> NSPLHTVGFDARFPQQNQTKHCWQSYVDYHKCVNMKGEDFAPCKVFWKTYNALCPLDWIEKWDDQREKGIFAGDINS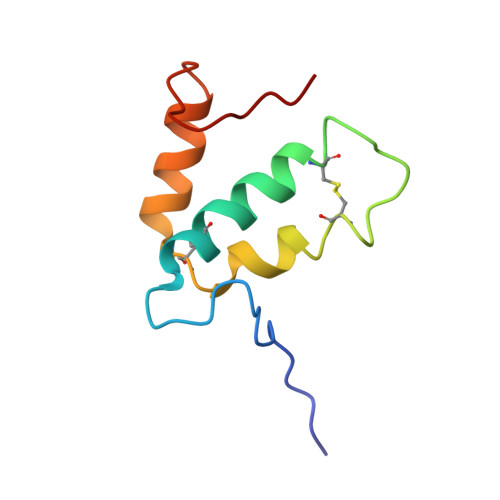D3,6-Bis{3-[(2R)-(2-ethylpiperidino)]propionamido}acridine | C33 H45 N5 O2 | 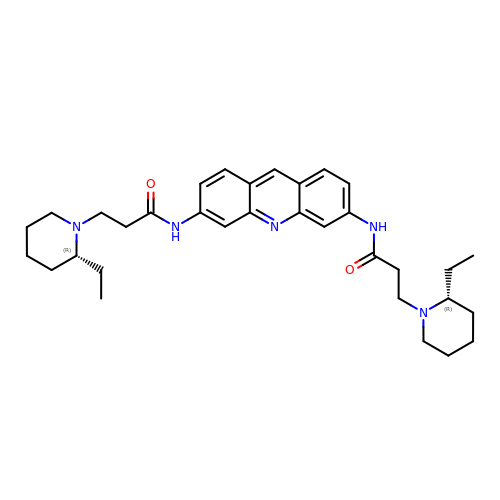ZWPUGYBFVBXUSX-FQLXRVMXSA-N>[2x]GSHMSLDNKPIMRVASIDIGSYSVRLTIAQIKDGKLSIILERGRITSLGTKVKETGRLQEDRIEETIQVLKEYKKL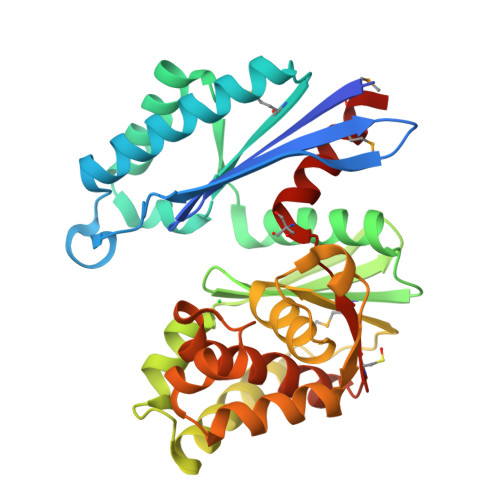IDEFKVERMKAVATEAIRRAKNAEEFLERVKREVGLVVEVITPEQEGRYAYLAVAYSLKPEGEVMVVDQGGGSTEYVFGKGYKVREVISLPIGIVNLTETFFKQDPPTEEEVKRFFEFLEKELSKVKKPVDTIVGLGGTITTLAALEYNVYPYDPQKVHGKVLTYGQIKKWFDTFKEIPSEERSKRFRQVEDRRAKVILAGIGIFLKTLEIFEKDCLIVSDWGLREGVLVSEMLKENHS>[4x]GALRGGMTSQLNELVEFLHSPQPAVRQIAIDNLVGFSAGPTSKVFKNDSYRPIKDIIKMIMDPEHGTRVIIQQGVTILVNLSEDKLVRNIILSDDKKFLKFLVWKIVDLTNPNADIMCILLSNLAKDDGILAVLNIKRNSSGEEVDDGLKLAALNKEVFKSLRAMDCLMDCFVKGYDKKLTKYASFNYLAFFFADISRFKLGRMYFIEEQEYDGVVPISKLLVFT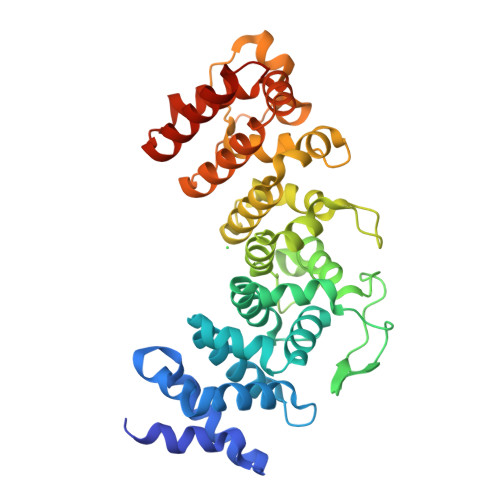EKYDAKVRREGVASTIKNSLFDSETHERLLKDEKINLLPYILLPIASAKDSEIDEEDMFNLPDELQLLPEDKERDPIPAIICCHLESILLLCTTHAGREYLRDKSVYPLVRELHKNVENEDIGELCYRIVNMLMRGEPGAGAVE>[2x]VDSVYRTRSLGVAAEGLPDQYADGEAARVWQLYIGDTRSRTAEYKAWLLGLLRQHGCQRVLDVACGTGVDSIMLVEEGFSVTSVDASDKMLKYALKERWNRRHEPAFDKWVI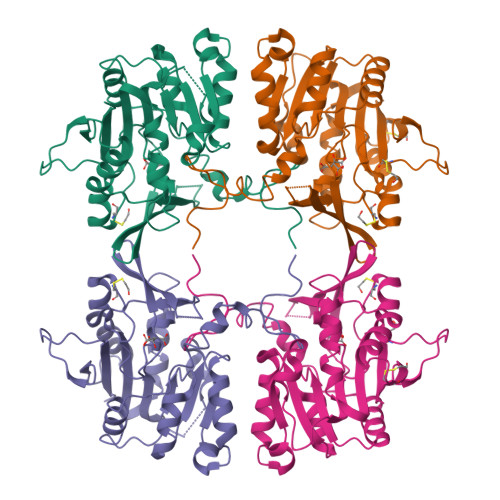EEANWMTLDKDVPQSAEGGFDAVICLGNSFAHLPDCKGDQSEHRLALKNIASMVRAGGLLVIDHRNYDHILSTGCAPPGKNIYYKSDLTKDVTTSVLIVNNKAHMVTLDYTVQVPGAGQDGSPGLSKFRLSYYPHCLASFTELLQAAFGGKCQHSVLGDFKPYKPGQTYIPCYFIHVLKRTD>[2x]MAVLGLQGVRGGVGTTTITAALAWSLQMLGENVLVVDACPDNLLRLSFNVDFTHRQGWARAMLDGQDWRDAGLRYTSQLDLLPFGQLSIEEQENPQHWQTRLSDICSGLQQLKASGRYQWILIDLPRDASQITHQLLSLCDHSLAIVNVDANCHIELHQQALPDGAHILINNFRIGSQVQDDIYQLWLQSQRRLLPMLIHRDEAMAECLAAKQPVGEYRSDALAAEEILTLANWCLLNYSGLKTPVGSKS;>[2x]GPMGSMNNNEPDTLPDPAIGYIFQNDIVALKQAFSLPDIDYADISQREQLAAALKRWPLLAEFAQQK;>[2x]MGSAEIQPRSDEKRILSNVAVLEGAPPLSEHWQLFNNNEVLFNEARTAQAATVVFSLQQNAQIEPLARSIHTLRRQRGSAMKILVRENTASLRATDERLLLACGANMVIPWNAPLSRCLTM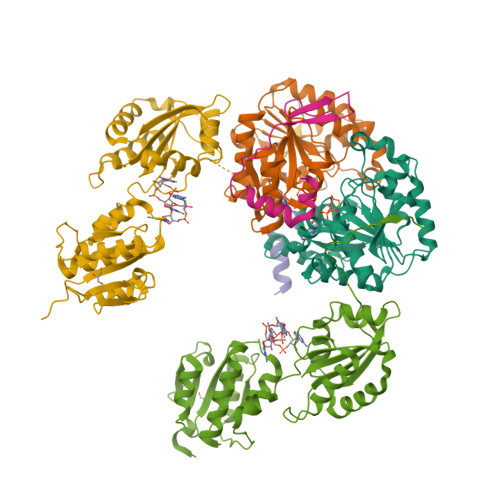IESVQGQKFSRYVPEDITTLLSMTQPLKLRGFQKWDVFCNAVNNMMNNPLLPAHGKGVLVALRPVPGIRVEQALTLCRPNRTGDIMTIGGNRLVLFLSFCRINDLDTALNHIFPLPTGDIFSNRMVWFEDDQISAELVQMRLLAPEQWGMPLPLTQSSKPVINAEHDGRHWRRIPEPMRLLDDAVERSS> SKPSKPFN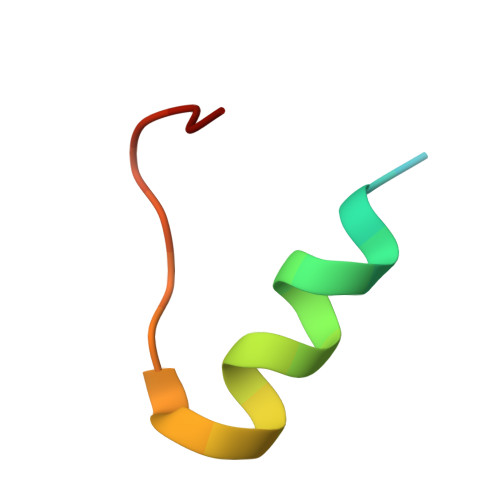VDDVLKFTFTGEKHHHHHH> HHHHHHTAQTVTGAVAAAQLGATLPHEHVIFGYPGYAGDVTLGPFDHAAALASCTETARALLARGIQTVVDATPNDCGRNPAFLREVSEATGLQILCATGFYYEGEGATTYFKFRASLGDAESEIYEMMRTEVTEGIAGTGIRAGVIKLASSRDAITPYEQLFFRAAARVQRETGVPIITHTQEGQQGPQQAELLTSLGADPARIMIGHMDGNTDPAYHRETLRHGVSIAFDRIGLQGMVGTPTDAERLSVLTTLLGEGYADRLLLSHDSIWHWLGRPPAI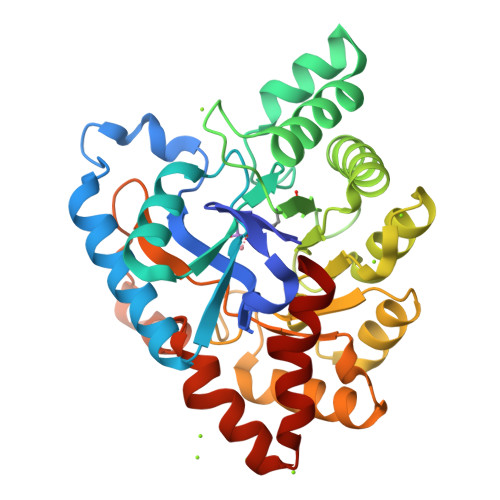PEAALPAVKDWHPLHISDDILPDLRRRGITEEQVGQMTVGNPARLFG> MGPGLLYNHAAKTAVNGIDRSTEGTNVSARLCNNISAVTFVSKYKAVCQPIADQLDLPVENLLGLAAQESQYGTGRIARELNNYFSMHAPAPLQIG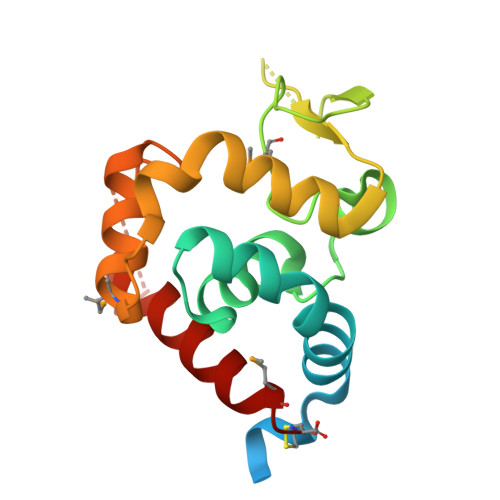AEAPLGNASIKVAKFDSFQKSAQSFASSFGTAVRGQRDPMAFAQALVRSGYNTGNAKTGGRDGFARYLADIIIAVRGRMAC>MKMLEQLEKKLGYTFKDKSLLEKALTHVSYSKKEHYETLEFLGDALVNFFIVDLLVQYSPNKREGFLSPLKAYLISEEFFNLLAQKLELHKFIRIKRGKINETIIGDVFEALWAA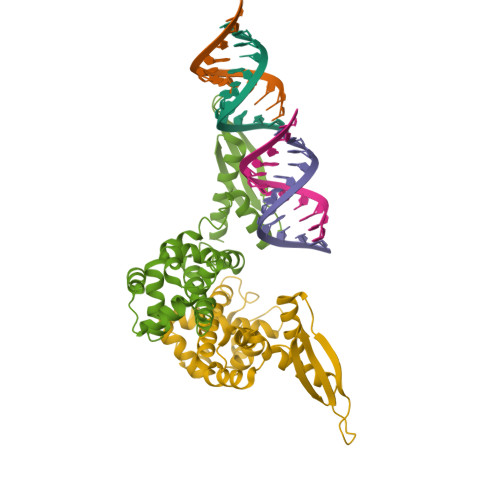VYIDSGRDANFTRELFYKLFKEDILSAIKEGRVKKDYKTILQEITQKRWKERPEYRLISVEGPHHKKKFIVEAKIKEYRTLGEGKSKKEAEQRAAEELIKLLEESE[4x]(S)-2-HYDROXY-2,3-DIMETHYLBUTANENITRILE | C6 H11 N O | 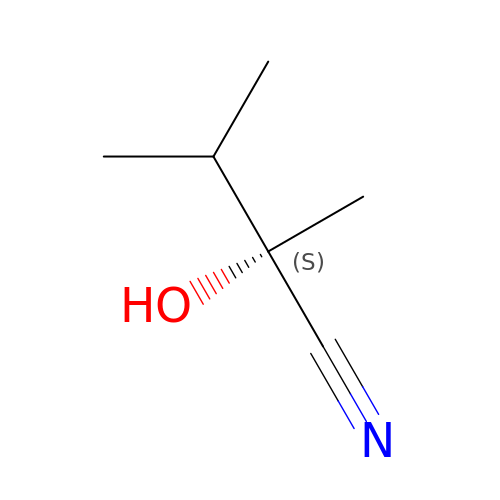QCKRFEBWZBKGTR-ZCFIWIBFSA-N4-[(6-CHLORO-2-NAPHTHALENYL)SULFONYL]-1-[[1-(4-PYRIDINYL)-4-PIPERIDINYL]METHYL]-2-PIPERAZINECARBOXYLIC 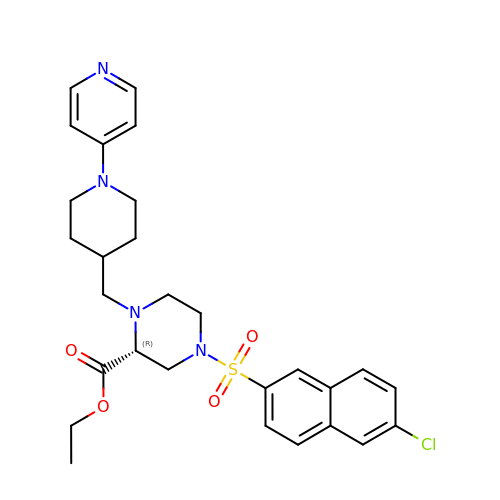ACID ETHYL ESTER | C28 H33 Cl N4 O4 S | KTOZABIXRDAUJO-HHHXNRCGSA-N N-[VALINYL]-N'-[ADENOSYL]-DIAMINOSUFONE 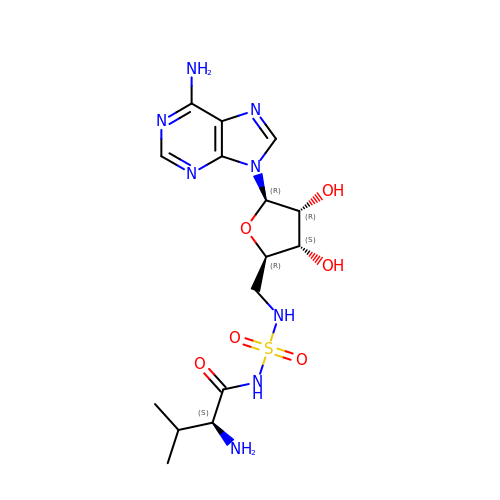| C15 H24 N8 O6 S | ILBDFTSSTCBHRF-CYUGOOACSA-N> MHHHHHHLVPRGSVHHIKRRDIVLKWELGEGAFGKVFLAE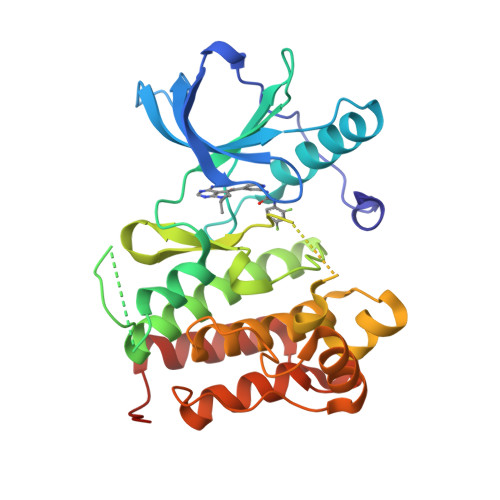CHNLLPEQDKMLVAVKALKEASESARQDFQREAELLTMLQHQHIVRFFGVCTEGRPLLMVFEYMRHGDLNRFLRSHGPDAKLLAGGEDVAPGPLGLGQLLAVASQVAAGMVYLAGLHFVHRDLATRNCLVGQGLVVKIGDFGMSRDIYSTDYYRVGGRTMLPIRWMPPESILYRKFTTESDVWSFGVVLWEIFTYGKQPWYQLSNTEAIDCITQGRELERPRACPPEVYAIMRGCWQREPQQRHSIKDVHARLQALAQAPPVYLDVLG In this work, we exhaustively probe the ability of all 36 immobile HJ sequences to form DNA crystals in two different designed systems. Three separate self-assembling DNA crystal systems are described in this report: the “4 × 5” and “4 × 6” designs (collectively referred to as the 4 × N systems), and a third construct with a “scrambled” sequence variant of the 4 × 6 lattices. Self-assembly was mediated by three constituent oligonucleotides: (S1) containing four sequence repeats of either 5 or 6 bases; (S2) composed of 21 bases containing complementary regions to both (S1); and (S3) which forms the second junction crossover. The HJ serves as the fundamental component at the core of each unit, and the ultimate assembly of the full lattice is facilitated by the complementary 2-base sticky ends that tail each duplex.

Each asymmetric unit could be defined as either a HJ containing 10 and 11 bp on each arm, or as a 21-bp linear duplex. The 4 × 5 system robustly crystallized with 75% of the junctions, and we obtained crystals in all but 9 of 36 sequences. Pos1 and 2 were readily observable in the electron density maps at either one or both of these conserved sites in a significant number of the structures, with no apparent respect to motif or symmetry.

> GAGCAGACTAGACACCACTCA;> TGTCT;> TCTGAGTGG;> AGTCTGC> TVKSGLILQSISNDVYHNLAVEDWIHDHMNLEGKPVLFLWRNSPTVVIGRHQNPWQECNLNLMREEGVKLARRRSGGGTVYHDMGNINLTFFTTKKKYDRMENLKLVVRALKAVHPHLDVQATKRFDLLLDGQFKISGTASKIGRNAAYHHCTLLCGTDGTFLSSL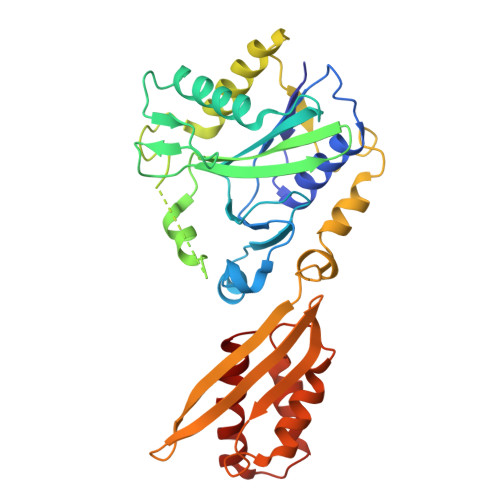LKSPYQGIRSNATASTPALVKNLMEKDPTLTCEVVINAVATEYATSHQIDNHIHLINPTDETVFPGINSKAIELQTWEWIYGKTPKFSVDTSFTVLHEQSHVEIKVFIDVKNGRIEVCNIEAPDHWLPLEICDQLNSSLIGSKFSPIETTVLTSILHRTYPGDDELHSKWNILCEKIKGIM>[3x]EELYQSILELKPLTLLMTSSTSFSETINQWADILKTTDMEKFSFDSNPINLLELVKQFNLYVD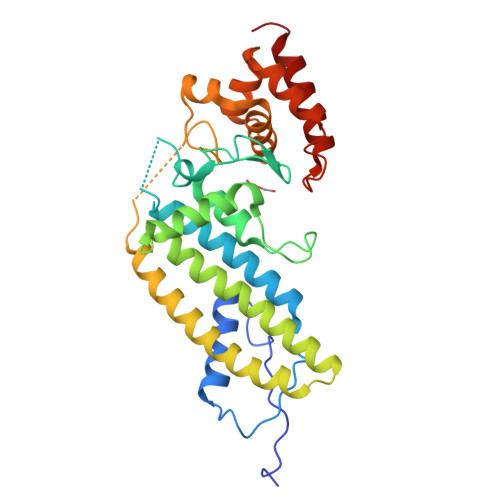ELAITCEANNVWAKERIDSTPNLFALYDNSGGEAIHGHAFVPYYKESIVLRRLFTVDPNTFNLSRFAAFEGPCQLYCAAHADSAWVKIQTLLTLGNGIINTLKIIKQAQAFGIDEAVTENLKALKEQFIAFQLAEADIKESLKAPSFAEPLPNKESEFFYPIDEKALAKMNGYQLATICLEELNSPKPSPLIERILSNKKFWKRINSAFESGVFKGRTDDPAGKIAKIREWHQLLQISG>[10x]NIEVLNLVTGPDSITTIELYLNTRMGQNDESKDNYGYSEKVTVANSSDQDKPTSGEIPTYSTARINLPMLNEDLTSNTLTMWEAVSVKTEVVGVSSLVNVHMATKRMYDDKGIGFPVEGMNFHMFAVGGEPLELQFLTGNYRTDYSANDKLVVPPIKHQSTQGLNPHYKQKLTKDGAFPVECWCPDPSKNENTRYYGSYTGGQSTPPVLQFTNTVTTVLLDENGVGPLCKGDGLYVSCCDI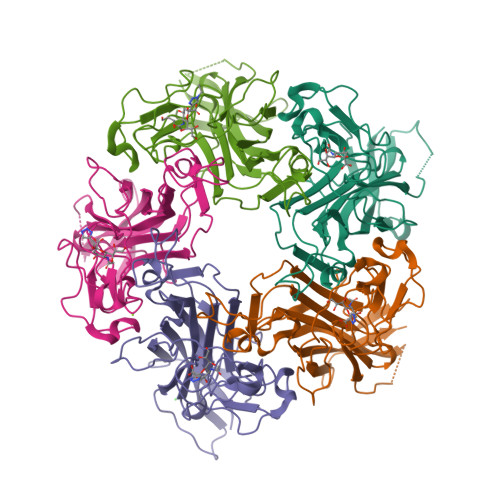VGFLVGKDGDMQYRGLPRYFNILLRKRTVRN> SNPCAKPHGKKLATVKQIAQYYKRKAYIQLNERGSRSALKGDASQGQYDRGGKADDFKTKLCEINEKHSNARSNSLNPCNGKDNNKVRFNVGTPWQSGEKIATATDVYLPPRRQHFCTSNLEYLINGGHQAILNVKNGKINHSFLGDVLLAAKYQAQHTMKDYKSKNDKEGICRAIRYSFADIGDIIKGTDLWDKDGGEIKTQNHLVTIFDKIKAQLPKDIKGKYTGTKHLELRKDWWEANRDQVWKAMQCGNDNPCSGESDHTPLHDYIPQRLRWMTEWAEWYCKEQSRLYDKLKVCEECMRKGESCTKGSGECATCKEACEEYNKEIKKWEQQWDAISYKYLMLYAKARITAINGGPGYYNTEVQEEDKPVVDFLYNLYLQNGGKKGPPPDTHRVKALIARVKRDAARNRVKRADGSSATRVTATTTITPYSTAAGYIHQEAHIGDCQKQTQFCKNKNGSDVSDTEADPTYAFRDKPHDHDTACKC;> QTSVSPSKVILPRGGSVLVTCSTSCDQPKLLGIETPLPKKELLLPGNNRKVYELSNVQEDSQPMCYSNCPDGQSTAKTFLTVYWTPERVELAPLPSWQPVGKNLTLRCQVEGGAPRANLTVVLLRGEKELKREPAVGEPAEVTTTVLVRRDHHGANFSCRTELDLRPQGLELFENTSAPYQLQTFG

Cerebral malaria is a deadly outcome of infection by Plasmodium falciparum, occurring when parasite-infected erythrocytes accumulate in the brain. These erythrocytes display parasite proteins of the PfEMP1 family that bind various endothelial receptors. Each Plasmodium falciparum genome contains ∼60 PfEMP1-encoding var genes, which can be classified according to their chromosomal context into groups A–E. They have large ectodomains containing multiple duffy binding-like (DBL) and cysteine-rich inter-domain region (CIDR) domains that can interact with specific human endothelial receptors. In particular, subclasses of DBLβ domains found in group A, B, and C PfEMP1 bind ICAM-1 (Bengtsson et al., 2013, Howell et al., 2008, Janes et al., 2011); CIDRα1 domains from group A PfEMP1 bind endothelial protein C receptor (EPCR) (Lau et al., 2015, Turner et al., 2013); and group B and C PfEMP1 contain CIDRα2–6 domains, which bind CD36 (Hsieh et al., 2016, Robinson et al., 2003). Here, we used structural biology to determine how a group of PfEMP1 proteins interacts with intercellular adhesion molecule 1 (ICAM-1), allowing us to predict binders from a specific sequence motif alone.

Of these, a complex of the PF11_0521 (PlasmoDB: PF3D7_1150400) DBLβ3_D4 domain and ICAM-1D1D2 formed crystals that diffracted to 2.8 Å resolution. The PF11_0521 DBLβ3_D4 domain adopts the classical DBL domain fold, consisting of a core of α helices, decorated by numerous loops. In contrast to previously characterized DBL domains, an extended α helix and a glycine and proline-rich linker form a unique feature that protrudes from the domain and generates part of the ICAM-1 interaction site. The DBLβ domain interacts with ICAM-1 through a complex, elongated binding interface that contains three distinct subsites with a total surface area of 1,144 Å2. Site 1 is formed from a patch of hydrophobic residues along one side of the extended α helix of DBLβ that interacts with a corresponding hydrophobic patch on the surface of ICAM-1 D1. Site 2 is formed by the subsequent linker of the DBLβ domain and forms hydrogen bonds with both ICAM-1 D1 and D2 domains. Site 3 is formed from part of a long loop that protrudes from the DBLβ domain and also contacts both ICAM-1 D1 and D2. The parts of this loop not in contact with ICAM-1 are not observed in the electron density, indicating flexibility. This loop is indeed predicted to be intrinsically disordered, but becomes partially ordered when bound to ICAM-1. By testing the eight residues that directly interact with ICAM-1, we found that each of the three subsites contains a critical residue that, when mutated, disrupts ICAM-1 binding.> MMTISDIIE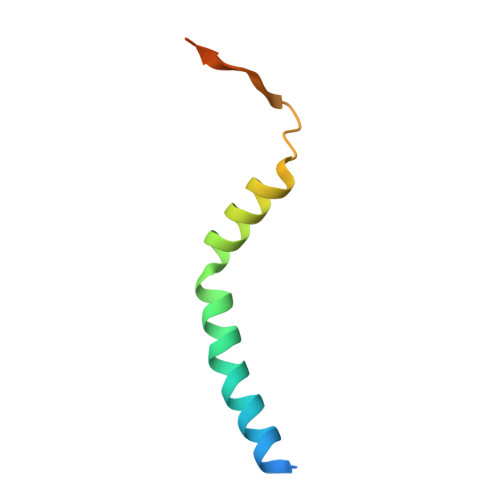IIVVCALIFFPLGYLARHSLRRIRDTLRLFFAKPRYVKPAGTLRRTEKARATKK>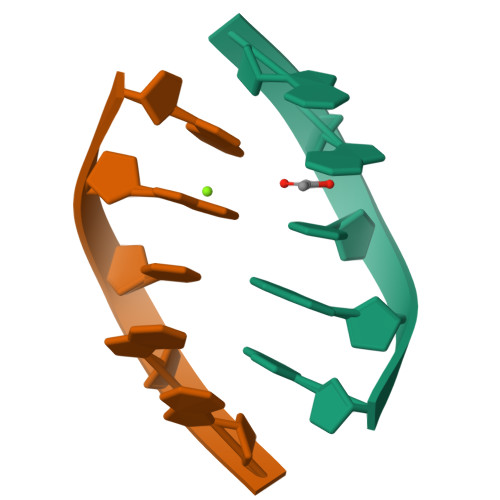AATGG[6x]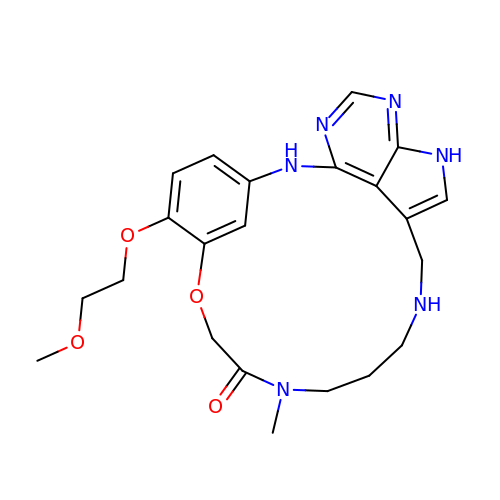6-(2-methoxyethoxy)-11-methyl-8-oxa-2,11,15,19,21,23-hexazatetracyclo[15.6.1.13,7.020,24]pentacosa-1(23),3(25),4,6,17,20(24),21-heptaen-10-one   | C22 H28 N6 O4 | MPVLMOBPNHBSRH-UHFFFAOYSA-N>[4x]SSYRQARWWAQEITELAQGPGRDFLQLHRHDSYAPPRPGTLARWFVNGAGYFAAVADAILRAQEEIFITDWWLSPEVYLKRPAHSDDWRLDIMLKRKAEEGVRVSILLFKEVELALGINSGYSKRALMLLHPNIKVMRHPDQVTLWAHHEKLLVVDQVVAFLGGLDLAYGRWDDLHYRLTDLGDSSESAASQPPTPRPDSPATPDLSHNQFFWLGKDYSNLITKDWVQLDRPFEDFIDRETTPRMPWRDVGVVVHGLPARDLARHFIQRWNFTKTTKAKYKTPTYPYLLPKSTSTANQLPFTLPGGQCTTVQVLRSVDRWSAGTLENSILNAYLHTIRESQHFLYIENQFFISCSDGRTVLNKVGDEIVDRILKAHKQGWCYRVYVLLPLLPGFEGDISTGGGNSIQAILHFTYRTLCRGEYSILHRLKAAMGTAWRDYISICGLRTHGELGGHPVSELIYIHSKVLIADDRTVIIGSANINDRSLLGKRDSELAVL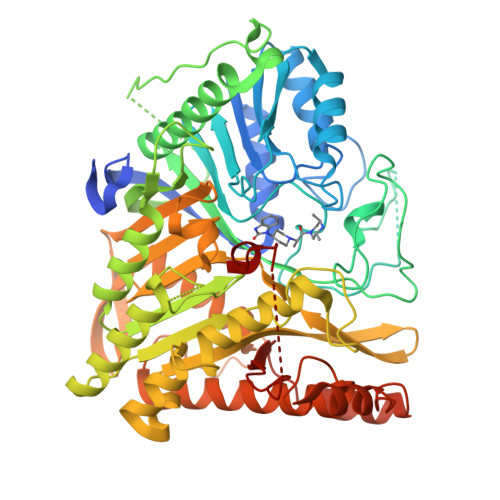IEDTETEPSLMNGAEYQAGRFALSLRKHCFGVILGANTRPDLDLRDPICDDFFQLWQDMAESNANIYEQIFRCLPSNATRSLRTLREYVAVEPLATVSPPLARSELTQVQGHLVHFPLKFLEDESLLPPLGSKEGMIPLEVWT N'-{(1S,2R)-1-(3,5-DIFLUOROBENZYL)-2-[(2R,4S)-4-ETHOXYPIPERIDIN-2-YL]-2-HYDROXYETHYL}-5-METHYL-N,N-DIPROPYLISOPHTHALAMIDE 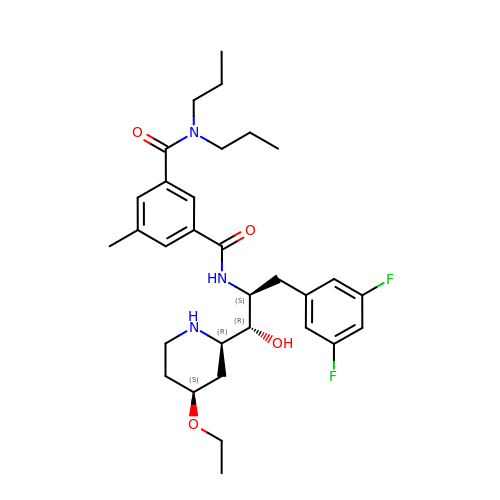| C31 H43 F2 N3 O4 | JWYOKBPWLVCFKU-ICYKMPLBSA-N> MAEQVALSRTQVCGILREELFQGDAFHQSDTHIFIIMGASGDLAKKKIYPTIWWLFRDGLLPENTFIVGYARSRLTVADIRKQSEPFFKATPEEKLKLEDFFARNSYVAGQYDDAASYQRLNSHMNALHLGSQANRLFYLALPPTVYEAVTKNIHESCMSQIGWNRIIVEKPFGRDLQSSDRLSNHISSLFREDQIYRIDHYLGKEMVQNLMVLRFANRIFGPIWNRDNIACVILTFKEPFGTEGRGGYFDEFGIIRDVMQNHLLQMLCLVAMEKPASTNSDDVRDEKVKVLKCISEVQANNVVLGQYVGNPDGEGEATKGYLDDPTVPRGSTTATFAAVVLYVENERWDGVPFILRCGKALNERKAEVRLQFHDVAGDIFHQQCKRNELVIRVQPNEAVYTKMMTKKPGMFFNPEESELDLTYGNRYKNVKLPDAYERLILDVFCGSQMHFVRSDELREAWRIFTPLLHQIELEKPKPIPYIYGSRGPTEADELMKRVGFQYEGTYKWVNPHKL

Reduced glutathione (GSH) provides the cellular first line of defense against oxidative stress-induced injury, which can be maintained by NADPH generated mainly via the pentose phosphate pathway and its rate-limiting enzyme, glucose-6-phosphate dehydrogenase (G6PD). Accordingly, missense DNA mutations that impair G6PD activity or stability result in increased oxidative stress and a spectrum of disease phenotypes featuring, most commonly, hemolytic anemia, and collectively called G6PD deficiency. Each monomer has a catalytic nicotinamide adenine dinucleotide phosphate (NADP+)-binding domain and β+α domain, containing an additional binding site for NADP+ that structurally stabilizes the enzyme. The glucose 6-phosphate (G6P)-binding site is located between these two domains.

To elucidate the molecular basis of the reduced stability and activity of Canton G6PD, we examined the crystal structures of WT and Canton G6PD at 1.9 Å and 2.6 Å resolution, respectively. Although no NADP+ was added to protein solution prior to the crystallization, both crystal structures contained NADP+ at the second NADP+-binding site (structural NADP+-binding site) in the β+α domain. The overall conformations of WT and Canton G6PD were very similar, as indicated by a root-mean-square deviation of 0.6 Å for the superimposition of Cα atoms. In WT G6PD, R459 forms electrostatic and hydrogen bond interactions with D181 and N185 on the adjacent helix (αe), whereas Canton mutation does not, resulting in loosened inter-helical interactions and displacements of the helix (αe) and a proceeding loop consisting of K171, P172, F173, G174, and R175, several amino acids away from R459-interacting residues on the helix (αe). In particular, K171 and P172 are the key residues involved in positioning of G6P and NADP+ in their binding pockets. We further mutated the R459-interacting residues, D181 and N185, to alanine in WT G6PD to determine the importance of the inter-helical interactions and found that these point-mutated enzymes are biochemically similar to the Canton variant; they exhibited about 20% of the normal activity, with lower KM values for both NADP+ and G6P and lower T1/2 values. Taken together, these data support the importance of the inter-helical interaction between R459 and D181 and N185 for catalytic activity and stability of the enzyme and provides a structural insight into the biochemical defects of the Canton variant.> MPFEVVFDGAKEFADLIATASNLIDEAAFKFTEEGISMRAMDPSRVVLIDLNLPESIFSKYEVEEPETIGINMDQFKKILKRGKAKDTLILRKGDENFLEITFEGTAKRTFRLPLIDVEELELELPELPFTAKVVL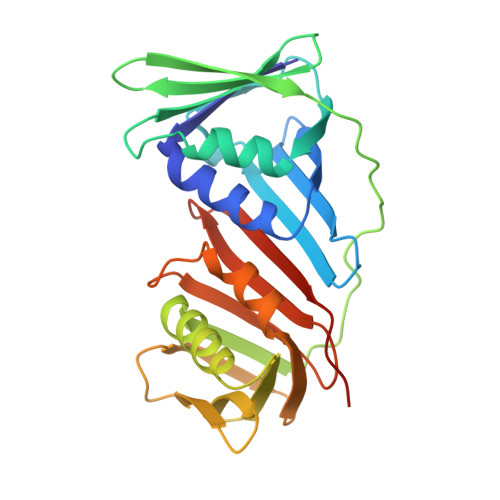LGEVLKEGIKDASLVSDAIKFIAKENEFTMKAEGETNEVEIRLTLEDEGLLDLEVEEETKSAYGIRYLSDMVKGIGKADEVILRFGNEMPLQMEYMIRDEGRLTFLLAPRVEEHHHHHH N-[1H-INDOL-3-YL-ACETYL]VALINE 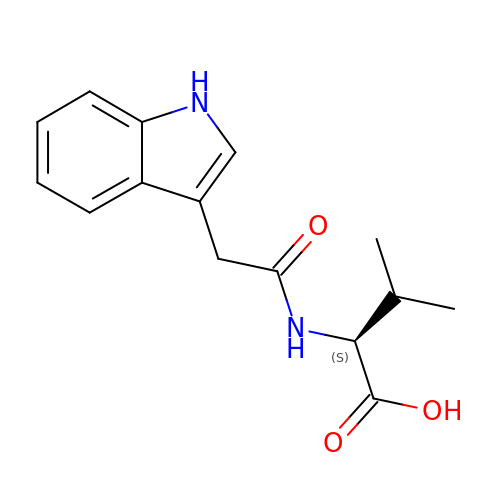ACID | C15 H18 N2 O3 | AZEGJHGXTSUPPG-AWEZNQCLSA-N>[5x]TTPHHISDVAIELFAAHGFTDVSVDDIARAAGIARRTLFRYYASKNAIPWGDFSTHLAQLQ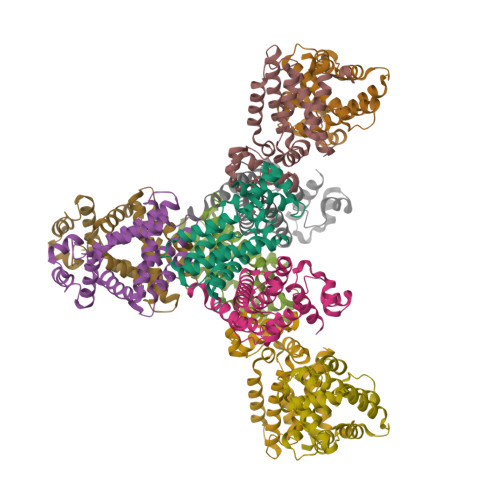GLLDNIDSRIQLRDALRAALLAFNTFDESETIRHRKRMRVILQTPELQAYSMTMYAGWREVIAKFVARRSGGKTTDFMPQTVAWTMLGVALSAYEHWLRDESVSLTEALGAAFDVVGAGLDRLNQ>GHMFESAEVGHSIDKDTYEKAVIELREALLEAQFELKQQARFPVIILINGIEGAGKGETVKLLNEWMDPRLIEVQSFLRPSDEELERPPQWRFWRRLPPKGRTGIFFGNWYSQMLYARVEGHIKEAKLDQAIDAAERFERMLCDEGALLFKFWFHLSKKQLKERLKALEKDPQHSWKLSPLDWKQSEVYDRFVHYGERVLRRTSRDYAPWYVVEGADERYRALTVGRILLEGLQAALATKERAKRQPHAAPLVSSLDNRGLLDSLDLGQYLDKDAYKEQLAAEQARLAGLIRDKRFRQHSLVAVFEGNDAAGKGGAIRRVTDALDPRQYHIVPIAAPTEEERAQPYLWRFWRHIPARRQFTIFDRSWYGRVLVERIEGFCAPADWL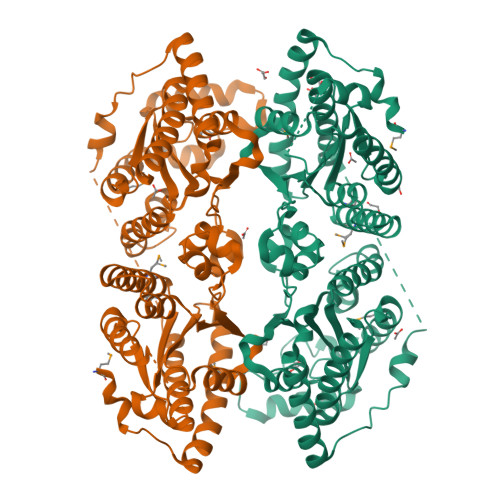RAYGEINDFEEQLSEYGIIVVKFWLAIDKQTQMERFKEREKTPYKRYKITEEDWRNRDKWDQYVDAVGDMVDRTSTEIAPWTLVEANDKRFARVKVLRTINDAIEAAYKKDKGA[2x]> MSAERTFLPNGNYNIKSIFSGSLYLSPVSGSLTFSNESSANNQKWNVEYMAENRCFKISNVAEPNKYLSYDNFGFISLDSL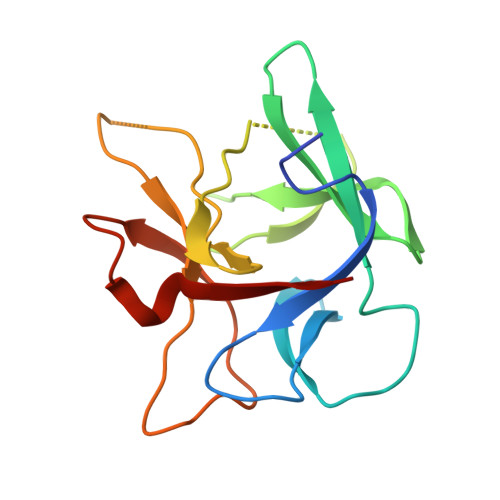SNRCYWFPIKIAVNTYIMLSLNKVNELDYAWDIYDTNENILSQPLLLLPNFDIYNSNQMFKLEKI>[2x]MGDKPIWEQIGSSFIQHYYQLFDNDRTQLGAI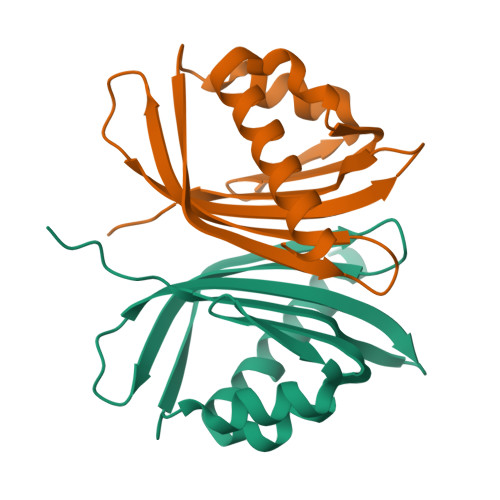YIDASCLTWEGQQFQGKAAIVEKLSSLPFQKIQHSITAQDHQPTPDSCIISMVVGQLKADEDPIMGFHQMFLLKNINDAWVCTNDMFRLALHNFG> SPSVEACGYSDRVAQLTVGNSSITTQEAANIVLAYGEWPEYCPDTDATAVDKPTRPDVSVNRFYTLDSKMWQENSTGWYWKFPDVLNKTGVFGQN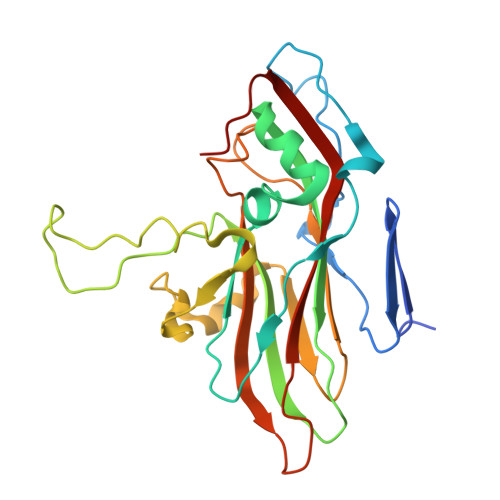AQFHYLYRSGFCLHVQCNASKFHQGALLVAVIPEFVIAGRGSNTKPNEAPHPGFTTTFPGTTGATFHDPYVLDSGVPLSQALIYPHQWVNLRTNNCATVIVPYINAVPFDSAINHSNFGLVVVPVSPLKYSSGATTAIPITITIAPLNSEFGGLRQAVSQ The glycosyltransferase WaaG in Pseudomonas aeruginosa (PaWaaG) is involved in the synthesis of the core region of lipopolysaccharides. The hexosyl sugar residue in each of the bacterial species is transferred by a glycosyltransferase (GT) referred to as WaaG to form an α-(1→3)-linkage. The PaWaaG monomer displays a typical GT-B fold, consisting of two “Rossmann-like” β/α/β domains.

In order to gain insights into substrate binding in PaWaaG we solved structures of the enzyme in complex with the nucleotide sugars UDP-glucose, UDP-galactose, and UDP-GalNAc in space group P21 to resolutions of 1.95, 2.02, and 2.20 Å, respectively. The PaWaaG-UDP-glucose and PaWaaG-UDP-GalNAc structures on the other hand, only have clear electron density for the relevant nucleotide sugars in one monomer and the second monomer is modeled with UDP only. Inspection of the substrate-binding site shows that the UDP component of the nucleotide sugars superimposes well with UMP from the PaWaaG-UMP structure, as exemplified with PaWaaG-UDP-glucose. In PaWaaG-UDP-glucose there are three hydrogen bond interactions (Glu281, Thr283, and Asn282) which position glucose, whereas there are two additional hydrogen bond interactions (Asp19 and the backbone nitrogen of Ala99) which orient galactose and GalNAc in the PaWaaG-UDP-galactose and PaWaaG-UDP-GalNAc structures, as well as the side-chain nitrogen atom of Asn282 which is in hydrogen bonding distance (3.1 Å) to O4′ of Gal and GalNAc. Interestingly, structural comparisons show that, while the galactose portion of PaWaaG-UDP-galactose superimposes perfectly with the galactose component of GalNAc from PaWaaG-UDP-GalNAc, it occupies a quite different position to the glucose moiety of PaWaaG-UDP-glucose. An interesting point of difference between the structures is the large difference in the binding modes of the glucose and 2F-glucose sugar moieties. In PaWaaG the glucose group is twisted significantly relative to 2F-glucose in EcWaaG, and is supported by hydrogen bonding with the sidechains of Glu281, Asn282, and Thr283. As EcWaaG specifically hydrolyzes UDP-glucose, the EcWaaG-UDP-2F-glucose structure represents productive substrate binding and we therefore speculated that our PaWaaG-UDP-glucose structure indicates nonproductive substrate binding. Solution state NMR experiments revealed that PaWaaG specifically hydrolyzes UDP-GalNAc and that the enzyme binds UDP-glucose but does not hydrolyze it. This indicates that our UDP-GalNAc structure represents productive substrate binding and confirms that the PaWaaG-UDP-glucose structure shows a nonproductive substrate binding mode.

> MATLAFILYKYFPFGGLQRDFMRIALECQRRGHDIRVYTLIWEGDVPDGFEVLVAPVRSIFNHRRNEKFTAWVRADLDRRPVQRVIGFNKMPGLDVYYAADACFEEKAQTLRNPLYRQWGRYRHFAGYERAVFDPASKTEILMISEVQQPLFVKHYGTQAERFHLLPPGISQDRRAPANAADVRAEFRREFGLEEDDLLLVQIGSGFKTKGLDRSLKALSALPKALRRRTRLIAIGQDDPKPFLLQIAALGLNDQVQILKGRSDIPRFLLGADLLIHPAYNENTGTVLLEALVSGLPVLVTDVCGYAHYIAEADAGRVLPSPFEQDSLNRLLAEMLEDAPARAAWSRNGLAYADHADLYSMPQRAADLILGEAS;> ATLAFILYKYFPFGGLQRDFMRIALECQRRGHDIRVYTLIWEGDVPDGFEVLVAPVRSIFNHRRNEKFTAWVRADLDRRPVQRVIGFNKMPGLDVYYAADACFEEKAQTLRNPLYRQWGRYRHFAGYERAVFDPASKTEILMISEVQQPLFVKHYGTQAERFHLLPPGISQDRRAPANAADVRAEFRREFGLEEDDLLLVQIGSGFKTKGLDRSLKALSALPKALRRRTRLIAIGQDDPKPFLLQIAALGLNDQVQILKGRSDIPRFLLGADLLIHPAYNENTGTVLLEALVSGLPVLVTDVCGYAHYIAEADAGRVLPSPFEQDSLNRLLAEMLEDAPARAAWSRNGLAYADHADLYSMPQRAADLILG>MAEMATATRLLGWRVASWRLRPPLAGFVSQRAHSLLPVDDAINGLSEEQRQLRQTMAKFLQEHLAPKAQEIDRSNEFKNLREFWKQLGNLGVLGITAPVQYGGSGLGYLEHVLVMEEISRASGAVGLSYGAHSNLCINQLVRNGNEAQKEKYLPKLISGEYIGALAMSEPNAGSDVVSMKLKAEKKGNHYILNGNKFWITNGPDADVLIVYAKTDLAAVPASRGITAFIVEKGMPGFSTSKKLDKLGMRGSNTCELIFEDCKIPAANILGHENKGVYVLMSGLDLERLVLAGGPLGLMQAVLDHTIPYLHVREAFGQKIGHFQLMQGKMADMYTRLMACRQYVYNVAKACDEGHCTAKDCAGVILYSAECATQVALDGIQCFGGNGYINDFPMGRFLRDAKLYEIGAGTSEVRRLVIGRAFNADFH[4x]

Isovaleryl-CoA (coenzyme A) dehydrogenase (IVD) is an intramitochondrial flavoenzyme that catalyzes the conversion of isovaleryl-CoA (3-methylbutyryl-CoA) into 3-methylcrotonyl-CoA in the leucine catabolism pathway, transferring electrons to the electron-transferring flavoprotein (ETF). Consistent with other ACADs, including short-, medium-, and long-chain ACADs, IVD is characterized by a tetrameric architecture composed of 4 identical subunits. Each subunit of IVD contains one noncovalently attached FAD molecule, imparting a characteristic yellow color to the purified enzyme. Dysfunction of IVD is linked to isovaleric acidemia (IVA), a rare metabolic disorder characterized by the accumulation of toxic metabolites.

During purification, the protein sample exhibited a conspicuous yellow color, indicative of its interaction with FAD, a cofactor that accepts electrons and stabilizes the conformation of IVD. Thus, the original structure of IVD was resolved in the form of only combining with FAD molecules, achieving a resolution of 2.55 Å. To enhance protein stability for cryo-EM analysis, additional FAD was incorporated into the sample buffer. Each tetramer of IVD can bind 4 FAD molecules. The base of the binding pocket, where the isoalloxazine ring of FAD resides, is predominantly composed of hydrophobic amino acids, while the opening toward the neighboring monomer accommodates the adenosine portion. The cryo-EM structure reveals that each FAD molecule is coordinated by residues from 2 adjacent monomers within the IVD tetramer. Specifically, T200 from one monomer forms hydrogen bonds with the isoalloxazine group of FAD, while Q323 from the neighboring monomer stabilizes the adenosine moiety. Other residues including R312, G384, T409, and E411, which interact with the ribose and pyrophosphate group, arise from bordering monomers as well. This inter-subunit binding mode implies that FAD not only participates in catalysis but also bridges monomers to facilitate tetramer assembly. Therefore, the binding of FAD also plays a critical role in stabilizing the protein structure, as validated by the modifications to the buffer system, where its addition reduced the protein’s propensity for precipitation.> MKHHHHHHHGAAGTSLYKKAGENLYFQGSHLQRNIYLSLLHMEPEEGQEKAPKVPDSVIRAALLRRAVEDIHRIIQIRTAKAACSTLLQRGSVGDDLWQRFLRAEKEMEDELRDVVMEANALVPGWGQIIFQSANEIAANKVLRDRLEEIEAQTARDKEWWEKRRATIKSEFMKELDAEEAVEK;> MSDLDTFTFIPLHIDPKSKAISAAPNALGTPSANKALETELAALNALHRALHTQIEGPIPVPPPPVPVNPKRSANINKLRESGNAEYRKQRYGDAIKLYTLGLQMALTRPAWEPAGLVRDEIHQLYSNRAQAYM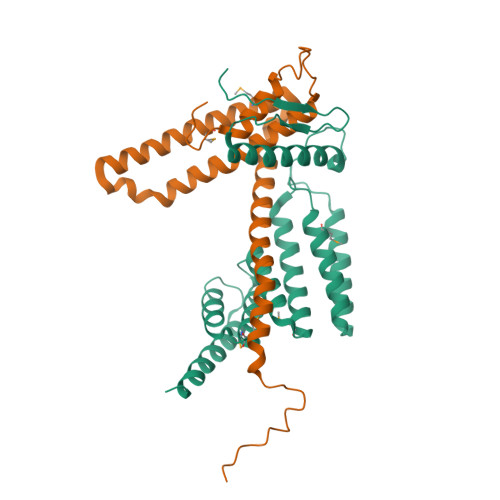QLGQWPEAAADAECSVEAKRQGNAKAWYRRGKCLMEMRRLQEAREWVARGLEFEGEEKELAELLKEIDSKLAAEKASRDA> SMGRLILEHTLQGHKGRIWGVAWHPKGNVFASCGEDKAIRIWSLTGNTWSTKTILSDGHKRTIREIRWSPCGQYLASASFDATTAIWSKSSGEFECNATLEGHENEVKSVSWSRSGGLLATCSRDKSVWIWEVAGDDEFECAAVLNPHTQDVKRVVWHPTK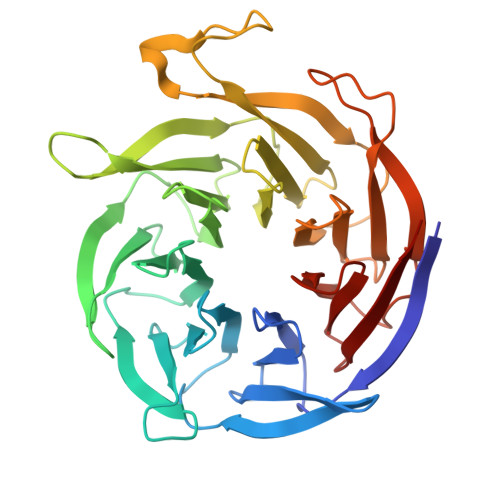DILASASYDNTIKMFAEEPIDNDWDCTATLTSHTSTVWGIDFDADGERLVSCSDDTTIKIWRAYHPGNTAGVATPDQQTVWKCVCTVSGQHSRAIYDVSWCKLTGLIATACGDDGIRIFKESSDSKPDEPTFEQITAEEGAHDQDVNSVQWNPVVAGQLISCSDDGTIKIWKVTE> MAGMALARAWKQMSWFYYQYLLVTALYMLEPWER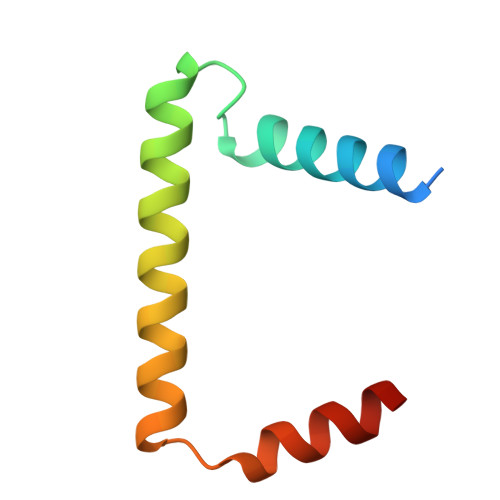TVFNSMLVSIVGMALYTGYVFMPQHIMAILHYFEIVQ4-chlorobenzyl carbamimidothioate | C8 H9 Cl N2 S 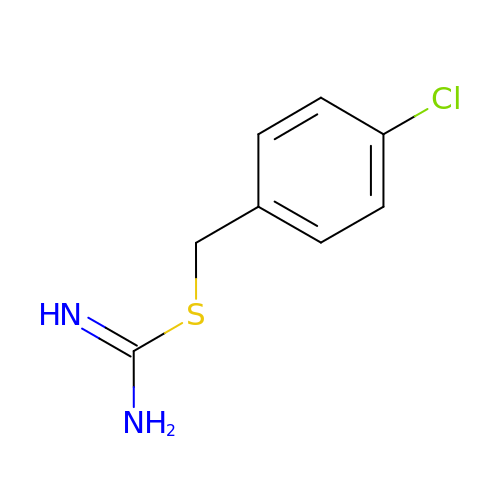| YOCWIHYZDHPSHD-UHFFFAOYSA-N>GHMTETKPRIAIRYCTQCNWLLRAGWMAQEILQTFASDIGEVSLIPSTGGLFEITVDGTIIWERKRDGGFPGPKELKQRIRDLIDPERDLGHVDRTKHEGLDTGS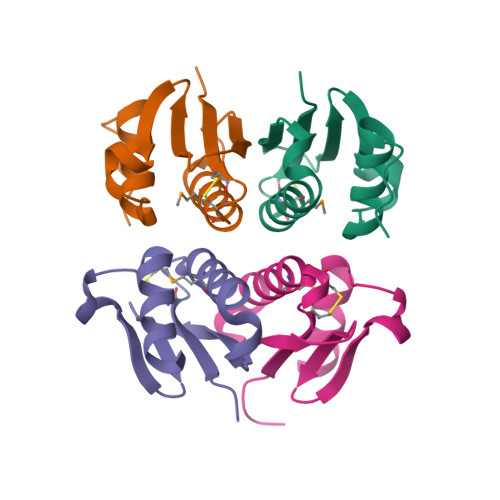[4x]>[2x]SNADPGAEPEASIDDLDAEALIRMALGPRNTMTSSNEQLVD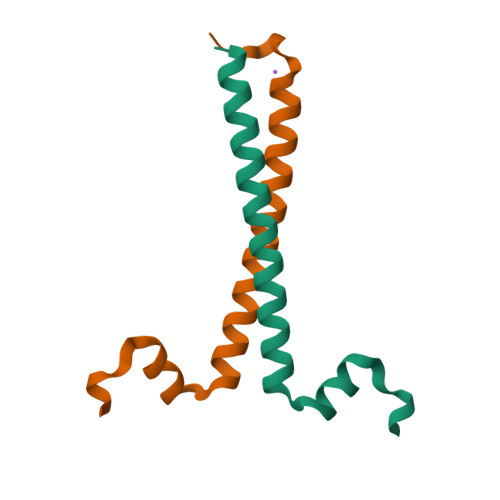ALRASLKENEELRKESRRRADRRQEPM>[4x]GSHMHRVINHPYYFPFNGKQAEDYLRSKERGDFVIRQSSRGDDHLAI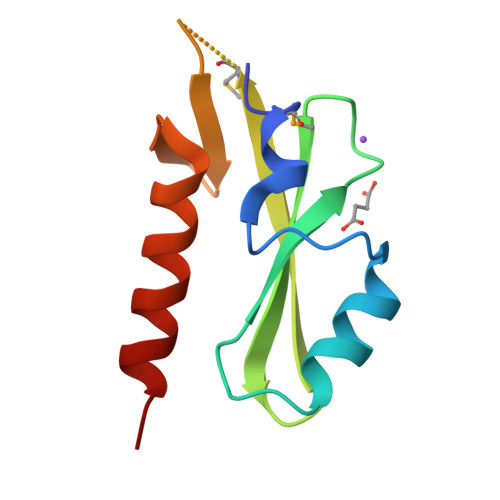TWKLDKDLFQHVDIQEMEKENPLAMGKVLVVEGQRYHDLDQIIVEYLQNKIRLLNE> GAMAAPAACTRFSDNYDIKEELGKGAFSIVKRCVQKSTGFEFAAKIINTKKLTARDFQKLEREARICRKLHHPNIVRLHDSIQEENYHYLVFDLVTGGELFEDIVAREFYSEADASHCIQQILESVNHCHQNGVVHRDLKPENLLLASKAKGAAVKLADFGLAIEVQGDHQAWFGFAGTPGYLSPEVLKKEPYGKSVDIWACGVILYILLVGYPPFWDEDQHRLYSQIKAGAY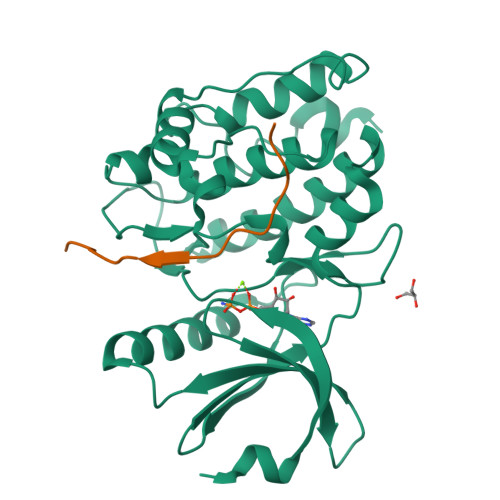DYPSPEWDTVTPEAKNLINQMLTVNPNKRITAAEALKHPWICQRERVASVVH;> GVLPKAPKLQASQATLARQDTIDEGGEVDSSPPSRDSRVVIEGAAVSSATVGPS> DCPSD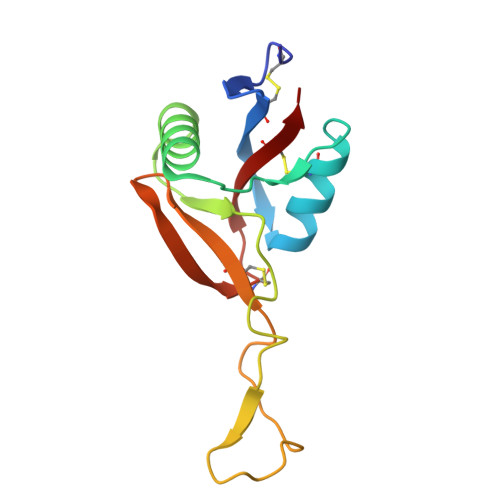WSSYEGHCYKPFNEPKNWADAENFCTQQHTGSHLVSFQSTEEADFVVKLAFQTFDYGIFWMGLSKIWNQCNWQWSNAAMLKYTDWAEESYCVYFKSTNNKWRSITCRMIANFVCEFQA>[2x]RKKVRKAVIPAAGLGTRFLP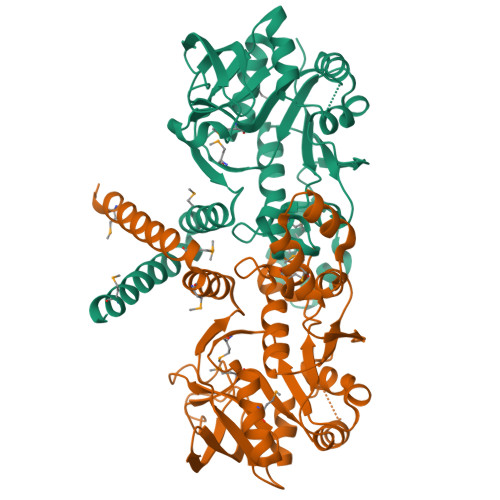ATKAQPKEMLPIVDKPAIQYIVEEAAESGIEDILIITGRNKRSIEDHFDRSAELEFNLREKGKTETLKEMQQIADLANIHYIRQKEPLGLGHAVLCAEHFIGDEPFAVLLGDDIMVSETPALRQLMDVYDVYGTEVVGVQSVLPEDVSKYGIINTSGSQGHVYEVNDLVEKPSPEEAPSEIAVMGRYVLNSSIFSVLKTIGRGAGNEIQLTDALREVCRKEPIHARLLEGNRYDIGDKLGCFKASTEIGLMRPEMRSQLLAYLEDVIKRETKEMLRL> TLLCGEIHYFRVPKHLWRDRLLKLKRAGGNCVSTYIPWNWHDPREKVVNFTDGTSQWHVASYYSRDLASFLELAGELGLRVIARPGPYICSEWDSGGHPNWIYTKAMRLRSLDPGYFKHVVEWYNSVLNILKPYVEREIVIGIQVENEYFWGNEKYIEKLAEIVEEKLPGVLVFTNEDPYLTRIPNTIDLYPSPWDMRQFDDRLRSYLSSQPGLFKMIMELEGGWFKSSRYGYYPTNRLSIPPEWTEILLKTAVGMGLNNINIYMFHGGSNPGYYTAKYLASSYDFEACIREWGELSERYYRVKRVFTFLNGFQELVTSLKPGETVKTASTCSELLQRVGDHGKIAVLRNTGDNLCYQRLINRGEIIPMWTPIRVPPRYAKIVLLDLVVEGTPFKLVYTSGEALLMKRLGDTVVMIIYGDHGEYTETAVEVEGGVLDVDIQGDVLIRREGERAYLVVNHTHGEHLAIVKSTRGQNLLLIFTCRCRAEKTWIVDEDLVLISNIYYIGDSRIDEGKVVINAELDEDSCGRLLVVTSREIEAISLEDLDLDLTRLSKYVYATHIPLSMCRSGKNTYHPLEYRLLEDPVFHTLTSINPSSPLLKNGFYENGIYVYRLRLHLDKKQLGDLLDKHLALI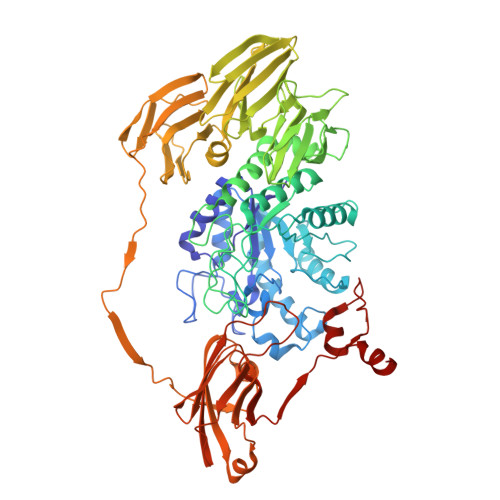GFSDYAVVSINNEYAGSGYHYIEMSADSLREGVNEVTVILESTGHPNDGLLYVPNGIYGGVYLGRVGEIRLYKWRKTGFEIPYGPGFDLAEFIANPEPVIKALQE>[8x]SNAYKMESRIKDISLAEFGLQDMEIAKTDMMGLVELQRKYRDSKPLKGARITGSLHLTIETSVLVETLYELGAEIRWCSCNIY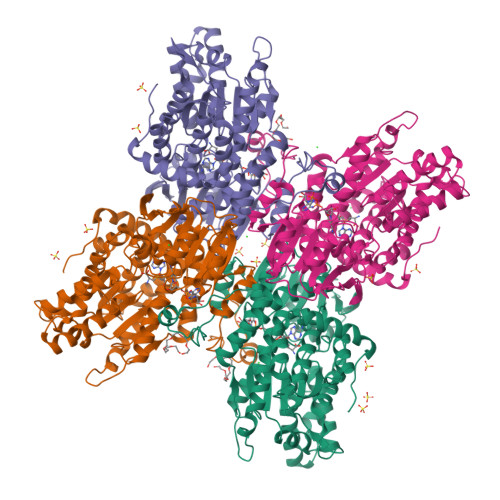STQDHAAAALVKKNIATVFAWKNETIEDYWVCLNDAMTWRNPNDKDKICGPNLIVDDGGDATLILHEGVKAEIEYEKYNKIPEYLETELDENGKQLSMDLKCMYKVLKMELLKNPFRWRGMLKDLYGVSEETTTGVLRLKIMESEGKLLLPAINVNDSVTKSKFDNTYGCRQSLLHGLFNGCIQMLAGKKIVVLGYGEVGKGCAQGLSGVGARVIVTEIDPICALQASMEGYQVSVLEDVVSEADIFITATGNKDVITVEHMRKMKENAYIANIGHFDDEIDVYGLENYPGIKVIEVKQNVHKFTFPDTQKSVILLCKGRLVNLGCATGHPPLVMSMSFTNQVLAQMDLWKSRELVDRSKNTRFFVKKLSKELDEYVARLHLDVLGIKLTKLTETQAKYINVSINGPYKSEDYRY>PEQNTWINRPEYSEVSEDRIVIVSDANTDFWENTYYDFSHYTGHVYGKETESDFTFQVRVKADFSALYDQAGIFIGGTETAWIKAGIEFNDGQPSIGCVVTNNNSDWSTGLFPGNPGDFWMRVTSKSDVIRIQYSIDGKNWPLLRLCTWPGTRKRFIGVMCCSPKRKGLSAEFTEIL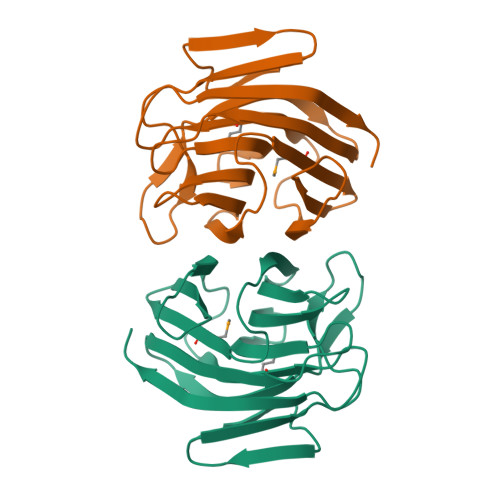LTTPLDSDLHDLSLEHHHHHH[3x]> MEKPTPLINSSMLGQYVGQTVRIVGKVHKVTGNTLLMQTSDLGNVEIAMTPDSDVSSSTFVEVTGKVSDAGSSF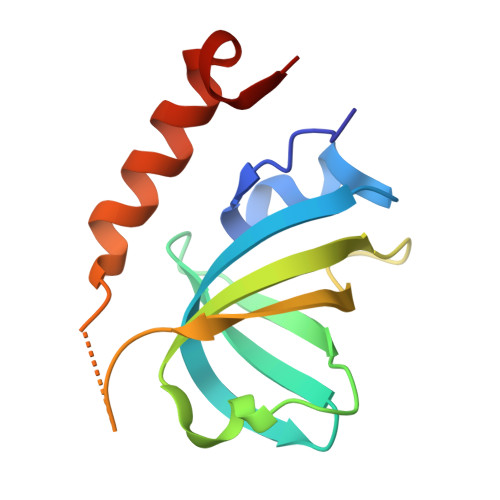QANQIREFTTVDCGHDVDLTLVENVVQISAAFPNLFSDST>[8x]MRHISPEELIALHDANISRYGGLPGMSDPGRAEAIIGRVQARVAYEEITDLFEVSATYLVATARGYIFNDANKRTALNSALLFLRRNGVQVFDSPELADLT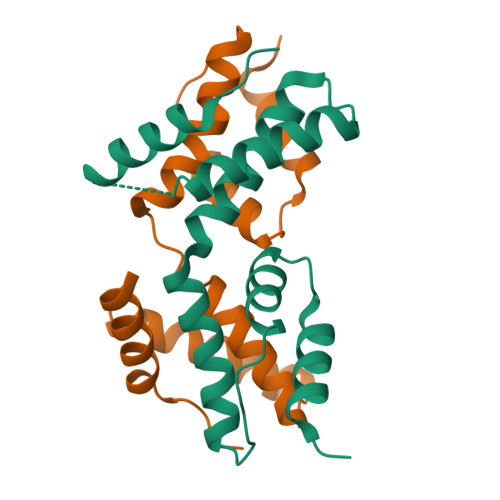VGAATGEISVSSVADTLRRLYGSADPLEHHHHHH N-{3-[4-(3-AMINO-PROPYL)-PIPERAZIN-1-YL]-PROPYL}-3-NITRO-5-(GALACTOPYRANOSYL)-ALPHA-BENZAMIDE | C23 H37 N5 O9 | 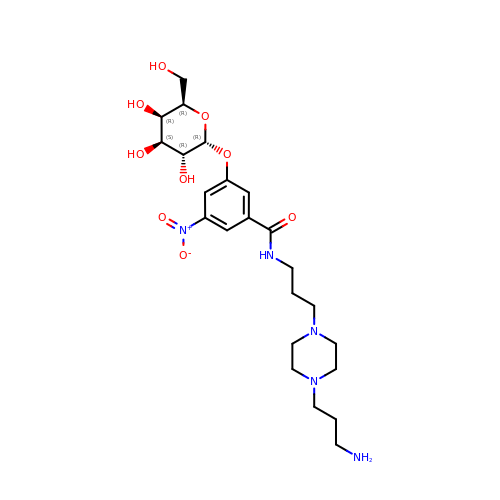UEIGEWJJVQHIAX-MKQKURRLSA-N> HHHHHHMEKTSAHVVPSMVRRNFCQLMTAATAAPFMGGALSAHAAAGHSAAFLKMDRSEEPSLLLRYDRSAANWNEALPIGNGRIGGMVWGNVSEEIIDLNEETLWSGHPRETDNPNAKQHLPQIRKAVFDKNYERANDLAYKIQGTYNENYQPLGQLHLSMSHAGESTNYARALDIGNAVSTVDYEVDGVKYHRDYFVSAPDNSMCIRLTASEPGKISCRLKMDSPLKHVSFSRGNSCIMQGQAPSHADRASIKADQVIFYDPKEEGLSFYSQLQVVPEGGRFWKYENGMRVEHADSLVLVFSAATNFDGFDVFPRKSRIDPCKVVKETFRKIGPVDFKELQKRHIADYRTLFDRVGIQLGKGASISKTTDQRIKDYARDEDPDLVALTFQYGRYMLISSSRPGTLPANLQGIWNPLMRPPWMSNWTNDLNTQMNYWLSWTTNLPECEKALIDWVDNLRPNGRKTARTNYGAKGWLCHNTTDLWMQTAPAGIERPRWCILPLGGVWLCQHLWMHYVFHGDREFLEKRSYPIMREAAEFCLDWLIKDSDGYYVTCPSVSPENWFATAGDKQLSISKASTYDMQLIRDLFTNCIQAAKVLNTDKEFSAKLQERMDHLYPQKIGQYGQLQEWSEDWDKPEDQHRHISHLFGLFPGDQLTPNKNPEGWKGARQSLLMRSGEMAKGGKGKNDADTGWSINWKIGWWARLHDAEQAQNMLRKIFRFAPSGNTLSSQKGGRYANLLNAGPPFQIDGVLGFTAGVVELLLQSHDGFIHLLPALPKNWPDGRVTGLKARGGFIVDIEWKDGKLLEAVIHPGHEKEVRVHYQDDVHVFAKIEKPVRITR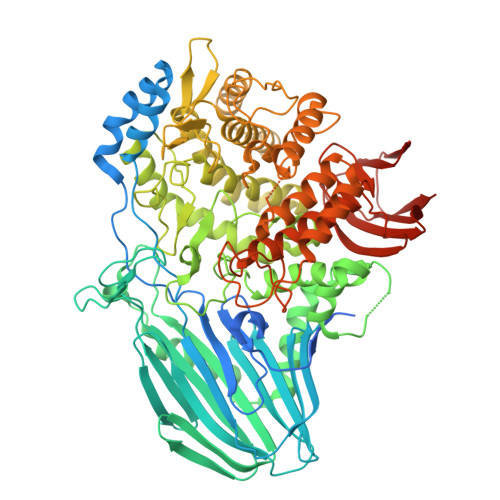HDHHHHHH> MTLHSWLDRYEKILASRGIKQKTLINYMSKI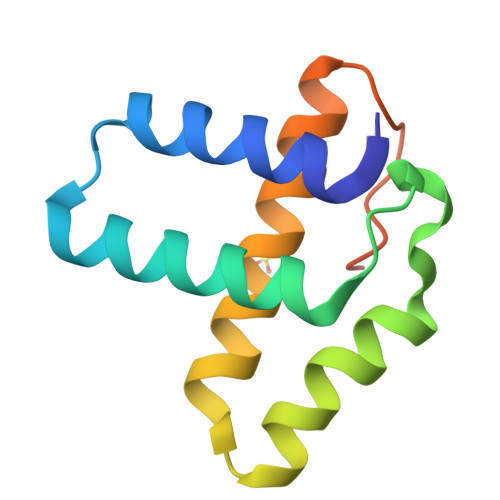KAIRRGLPDAPLEDITTKEIAAMLNGYIDEGKAASAKLIRSTLSDAFREAIAEGHITTNHVAATRAAKSEVR>MESTSTTVPSIVVYVTVPNKEAGKRLAGSIISEKLAACVNIVPGIESVYWWEGKVQTDAEELLI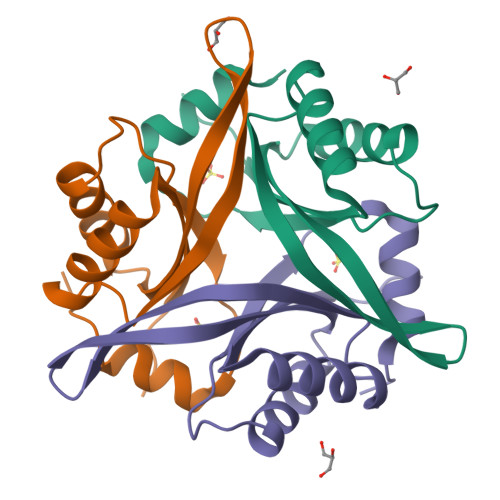IKTRESLLDALTEHVKANHEYDVPEVIALPIKGGNLKYLEWLKNSTRES[3x]>MAFSADTPEIVYTHDTGLDYITYSDYELDPANPLAGGAAWIEGAFVPPSEARISIFDQGFYTSDATYTTFHVWNGNAFRLGDHIERLFSNAESIRLIPPLTQDEVKEIALELVAKTELREAMVTVTITRGYSSTPFERDITKHRPQVYMSACPYQWIVPFDRIRDGVHLMVAQSVRRTPRSSIDPQVKNFQWGDLIRAIQETHDRGF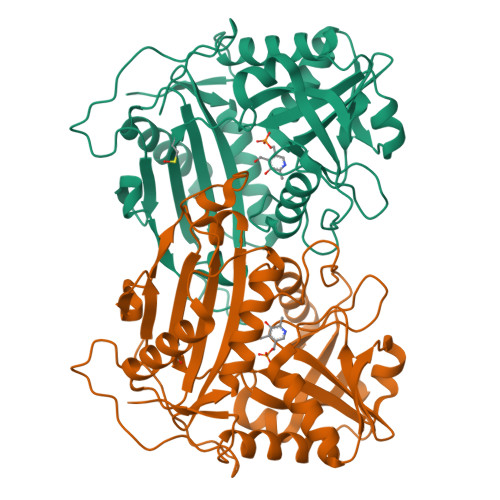ELPLLLDCDNLLAEGPGFNVVVIKDGVVRSPGRAALPGITRKTVLEIAESLGHEAILADITPAELYDADEVLGCSTGGGVWPFVSVDGNSISDGVPGPVTQSIIRRYWELNVEPSSLLTPVQY[12x]> GSGSSARHMVMQKLLRKQESTVMVLRNM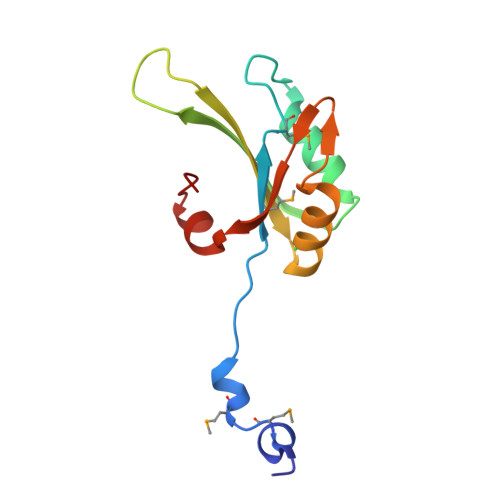VDPKDIDDDLEGEVTEECGKFGAVNRVIIYQEKQGEEEDAEIIVKIFVEFSIASETHKAIQALNGRWFAGRKVVAEVYDQERFDNSDLSA~{N}-[[2-(3-chloranyl-4-propan-2-yloxy-phenyl)pyrimidin-5-yl]methyl]-2-(trifluoromethyl)pyridin-4-amine | C20 H18 Cl F3 N4 O | 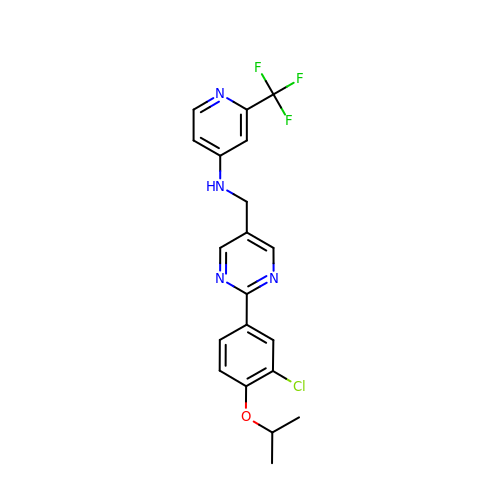FGUVKWPOHXVGKT-UHFFFAOYSA-N>MNTSNITFIGGGNMARNIVVGLIANGYDPNRICVTNRSLDKLDFFKEKCGVHTTQDNRQGALNADVVVLAVKPHQIKMVCEELKDILSETKILVISLAVGVTTPLIEKWLGKASRIVRAMPNTPSSVRAGA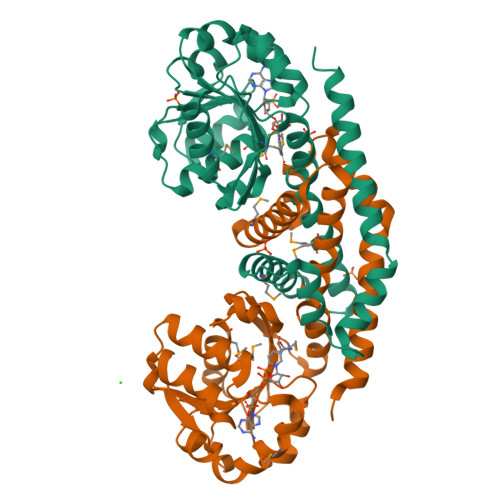TGLFANETVDKDQKNLAESIMRAVGLVIWVSSEDQIEKIAALSGSGPAYIFLIMEALQEAAEQLGLTKETAELLTEQTVLGAARMALETEQSVVQLRQFVTSPGGTTEQAIKVLESGNLRELFIKALTAAVNRAKELSKTVDQENLYFQ[2x]2-sulfanylideneimidazol-4-one | C3 H2 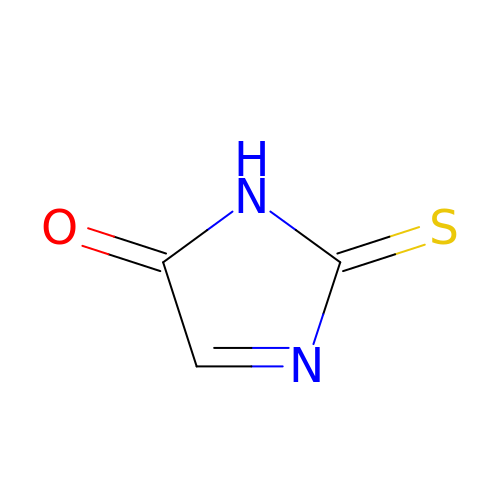N2 O S | KAKLKODZMNCHIC-UHFFFAOYSA-N>MSVVISDAWRQRFGGTARLYGEKALQLFADAHICVVGIGGVGSWAAEALARTGIGAITLIDMDDVCVTNTNRQIHALRDNVGLAKAEVMAERIRQINPECRVTVVDDFVTPDNVAQYMSVGYSYVIDAIDSVRPKAALIAYCRRNKIPLVTTGGAGGQIDPTQIQVTDLAKTIQDPLAAKLRERLKSDFGVVKNSKGKLGVDCVFSTEALVYPQSDGTVCAMKATAEGPKRMDCASGFGAATMVTATFGFVAVSHALKKMMAKAARQGLEHHHHHH[4x]

The enzyme responsible for t6A cyclization in E. coli was identified by comparative genomic approaches and analysis of LC/MS data sets of genomic deletion strains (ribonucleotide analysis) as CsdL, subsequently renamed to TcdA, for tRNA threonylcarbamoyladenosine dehydratase A. TcdA is an ubiquitin-activating E1-like protein with detectable homology to the adenylyltransferases MoeB and ThiF. To further the understanding of ct6A biology we have determined the high-resolution crystal structures of CsdL/TcdA in complex with AMP and ATP, an E1-like activating enzyme from Escherichia coli, which catalyzes the ATP-dependent dehydration of t6A to form ct6A. CsdL/TcdA is a dimer whose structural integrity and dimer interface depend critically on strongly bound K+ and Na+ cations. The tertiary structure of monomeric TcdA consists of seven β-strands in a continuous sheet surrounded by eight α-helices.

To shed light onto the structural basis for the tRNA binding and ct6A synthetic properties of TcdA-ATP, we determined the crystal structure of E. coli TcdA loaded with ATP to 1.77 Å resolution (R/Rfree values of 0.139/0.176) and AMP to 1.89 Å resolution (R/Rfree values of 0.141/0.183). The asymmetric unit contained four TcdA chains arranged in two independent dimers, with a solvent content of 39%. In the TcdA-ATP complex, ATP is bound in a cleft over the C-terminal end of the central sheet. The residues in the P loop form the floor of the nucleotide triphosphate moiety, and the adenine ring is inserted into a hydrophobic cavity. Specific interactions anchor ATP at the active site through its triphosphate moeity and the ribose hydroxyl groups. A short hydrogen bond between the main-chain carbonyl oxygen from the P-loop Gly40 maintains the α-phosphate group firmly bound insite the binding pocket in a kinked conformation. The conserved Arg72 and Lys85 contact oxygens from the α- and β-phosphates, while Thr68 and the strictly conserved Asn69 in the H310a helix anchor the γ-phosphate through a water-mediated hydrogen bond. In the TcdA-ATP and TcdA-AMP complexes, the region between β7 and the C-terminal α8 spanning residues 214–236 is fully disordered in electron density maps. Besides localized changes in the active site, the TcdA-ATP and TcdA-AMP structures are identical (RMSD 0.16 Å over 246 Cα atoms). The TcdA dimer is maintained by Na+, which mediates monomer-monomer contacts through the dimer interface, and by K+ ions, which play a structural role in shaping the monomer fold.Ups1 is located in the mitochondrial intermembrane space and is a member of the conserved UPS1/PRELI protein family, which is associated with mitochondrial function. Mdm35 is another conserved yeast intermembrane space protein belonging to the twin Cx9C protein family. As the binding partner of the Ups proteins, Mdm35 facilitates their mitochondrial import and protects them against proteolysis. The role of the Ups1/Mdm35 complex in lipid transfer was first reported in 2012; thereafter, Ups1 was recognized as a lipid transfer protein mediating PA shuttling between mitochondrial membranes.

To investigate the mechanism underlying Ups1/Mdm35-mediated PA transfer, we attempted to obtain the structure of PA-bound Ups1/Mdm35. Both Ups1/Mdm35 and Ups-Mdm35 fusion protein were co-crystallized with PA with different acyl chains, including 1,2-dioleoyl-sn-glycero-3-phosphate (DOPA; 18:1–18:1), 1-palmitoyl-2-oleoyl-sn-glycero-3-phosphate (POPA; 16:0–18:1), and 1,2-dihexanoyl-sn-glycero-3-phosphate (DHPA; 6:0–6:0). Although we obtained DOPA- and DHPA-bound Ups1/Mdm35 crystals, only DHPA-bound Ups1/Mdm35 crystals diffracted well. Two Ups1/Mdm35 molecules were present per asymmetric unit in Ups1/Mdm35–DHPA structure. The Ups1 molecules also form a domain-swapped dimer. In Ups1/Mdm35–DHPA structure, each Ups1/Mdm35 contains a DHPA molecule with high real-space correlation coefficients. Residues V66–G72 at the α2-loop could not be assigned because of a low electron density, suggesting the high flexibility of this loop. The phosphate head of bound DHPA is proximal to the positively charged R25 side chain, and the H33, K58, and N152 side chains are adequately proximal to facilitate electrostatic interactions or hydrogen bonds with the phosphate oxygen atoms. The sn-1 and sn-2 acyl chains of DHPA were stabilized via hydrophobic interactions with T76, I78, M104, and V106. Structural comparison of Ups1/Mdm35–DLPA and Ups1/Mdm35–DHPA revealed that DLPA is inserted deeper into the positively charged pocket than DHPA. However, in Ups1/Mdm35–DHPA, Mdm35 αA and αB helices interact with a Ups1 molecule, whereas its αC-helix interacts with another Ups1 molecule.

>[2x]MGNIMSASFAPECTDLKTKYDSCFNEWYSEKFLKGKSVENECSKQWYAYTTCVNAALVKQGIKPALDEAREEAPFENGGKLKEVDK;>[2x]MGSSHHHHHHSQDPMVLLHKSTHIFPTDFASVSRAFFNRYPNPYSPHVLSIDTISRNVDQEGNLRTTRLLKKSGKLPTWVKPFLRGITETWIIEVSVVNPANSTMKTYTRNLDHTGIMKVEEYTTYQFDSATSSTIADSRVKFSSGFNMGIKSKVEDWSRTKFDENVKKSRMGMAFVIQKLEEARNPQF>HHHHHHSSGLVPRGSHMTIFPDDFLWGGAVAANQVEGAYNEDGKGLSVQDVLPKGGLGEATENPTEDNLKLIGIDFYHKYKEDISLFSEMGFNVFRTSIAWSRIFPKGDEEEPNEAGLKYYDELFDELHAHGIEPLVTLSHYETPLYLARKYHGWVDRRMIHFYEKFARTVLERYKDKVKYWLTFNEVNSVLELPFTSGGIDIPKENLSKQELYQAIHHELVASSLVTKIAREINSEFKVGCMVLAMPAYPMTPNPKDVWATHEYENLNYLFSDVHVRGYYPNYAKRYFKENDINIEFAAEDAELLKNYTVDFLS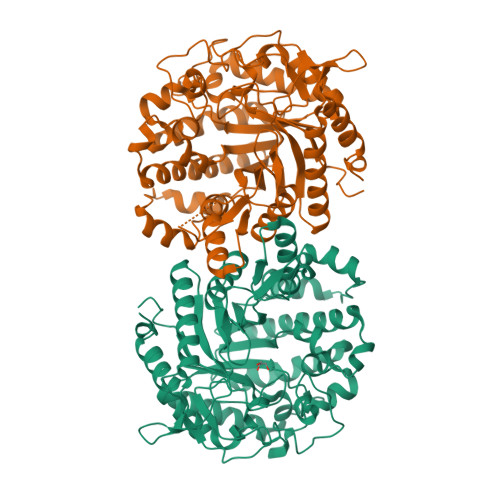FSYYMSVTQSALPTQYNSGEGNIIGGLVNPYLESSEWGWQIDPIGLRIILNRYYDRYQIPLFIVENGLGAKDQLIKDELNNLTVQDDYRIQYMKEHLLQVAEALQDGVEIMGYTSWGCIDCVSMSTAQLSKRYGLIYVDRNDDGSGTLNRYKKMSFTWYKEVIESNGESLFK[2x]Here we dissected the structural basis for neuropeptide-gated activity of a neuropeptide-gated DEG/ENaC, FMRFamide-gated sodium channel 1 (FaNaC1) from the annelid worm Malacoceros fuliginosus, using cryo-electron microscopy. We solved high-resolution structures of FaNaC1 alone, with full agonist FMRFa, with partial agonist ASSFVRIa, and with both FMRFa and pore-blocker diminazene, identifying the ligand-binding site and elucidating the conformational changes induced by ligand binding. Each subunit comprises a minimal N terminus and a nonresolved 63-amino acid C terminus facing the intracellular side, two transmembrane segments (TM1 and TM2), and a large extracellular domain. The FaNaC1 structures presented here capture a ligand-free resting state, two ligand-bound desensitized states and a ligand-bound dilated channel state.

We examined the structural basis of this partial agonism by solving the cryo-EM structure of FaNaC1 in the presence of ASSFVRIa, a product of the FVRIamide precursor in several annelids that gates FaNaC1 with relatively low potency and efficacy. The FaNaC1/ASSFVRIa cryo-EM map was resolved to 2.4 Å resolution, with a discrete density in the same ligand-binding pocket as that described for FMRFa. This density was best fit by the C-terminal FVRIa segment of the peptide, and the N-terminal ASS segment was not resolved. Full agonist FMRFa and partial agonist ASSFVRIa induce highly similar FaNaC1 conformations. In addition to the high similarity between FaNaC1/FMRFa and FaNaC1/ASSFVRIa structures, neither preparation yielded additional distinct 3D classes or any indication of conformational heterogeneity in the image processing. Thus, the partial agonism of ASSFVRIa does not appear to derive from the induction of a different conformational state compared to FMRFa. In both ligand-bound structures, however, the channel pore appears closed, with radii of ~1 Å at the level of G503 and G506 in TM2a (G3′ and G6′ in a TM2 numbering scheme). Thus, FMRFa- and ASSFVRIa-bound channels have probably adopted a desensitized state in the prolonged presence of agonist, in accord with the large decrease in current amplitude that occurs within ~2 s of FMRFa application, especially at higher FMRFa concentrations (for example).

>[3x]MSAIRDVMTKFAEQTTMHGVPKVINAKSSMGRLFWSLVCLAAGAMFCLQMSEVLQRYFSYPKKVTVEVVPTPVPFPSISICNMRNLDVHILNTLNRMFIEDDRPFSNINKSEHEFIRAYMKKVAKYAPLFWNYQDEYPEVFQEIFSRTTFSANIDPEVIALAAVQLEGFVVNCHYAGHRCNKTRDFYRFFDPYYFNCFTYKAHEPTDIEDNLSEGIENGWSSILLSGSGMLDKNDEIRMLPGLHEWRSAVSASEGVRVVIHPPSTTPYPFTEGYDVPPGFSASFGIHPRRNIRIGPPHGNCSDKNPFGDGTERYRLMACQKMCMQHYIVETCGCADVGLPKLPLQANISWCRDDDNFPDECMFTASEECLQLLMQLHNRIKCARSIKSKITKNTTAMEACNCFPPCDEVSYDVSYSLSKWPSAGYEGDAAYFDVFGIEKFNERFNKTGTQGKYELFTKYFNVSNREESMKDFARLNVYIADSNVVKTQESEDYTRNQLVSDIGGQLGLWVGISLITLAEVLELIIDLFRLFSKHTYRSVPVIRQSIKYKDKRNGAEMNYDTRYSQSNGGPHARYLHHGHSIPKHPPELPDTSLALEVLFQ;>ASSFVRIX[3x]>MSEWMKKGPLEWQDYIYKEVRVTASEKNEYKGWVLTTDPVSANIVLVNFLEDGSMSVTGIMGHAVQTVETMNEGDHRVREKLMHLF[2x];>[2x]AQESLESQEQRARAALRERYLRSLLAMVGHQVSFTLHEGVRVAAHFGATDLDVANFYVSQLQTPIGVQAEALLRCSDII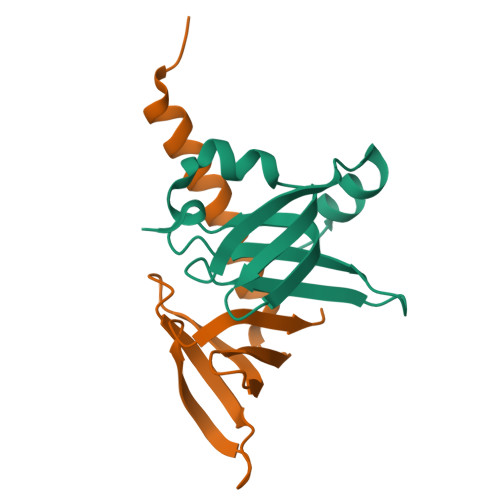SYTFKP N-acetyl-D-phenylalanyl-N-[(2S,3S)-6-carbamimidamido-1-chloro-2-hydroxyhexan-3-yl]-L-phenylalaninamide | C27 H38 Cl N6 O4 | 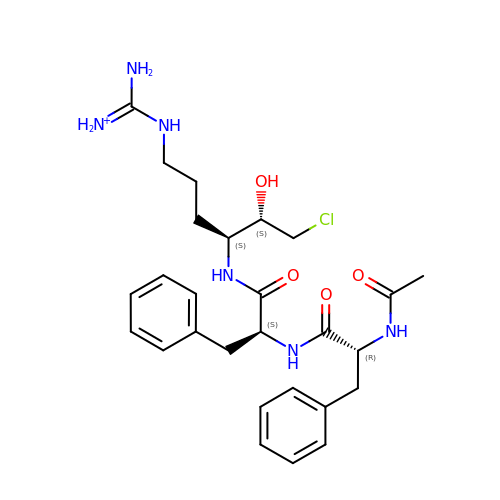SPENPXIFXGPVHG-UARRHKHWSA-O>[10x]DYKDDDDK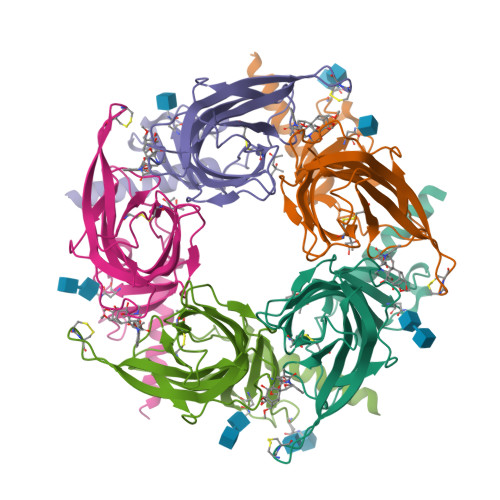LHSQANLMRLKSDLFNRSPMYPGPTKDDPLTVYLSFSLLDIVKADSSTNEVDLVYWEQQSWKLNSLMWDPNEYGNITDFRTSAADIWTPDITAYSSTRPVQVLSPQNALVNSSGHVQYLPAQRLSFMCDPTGVDSEEGATCAVKFGSWSYGGWEIDLKTDTDQVDLSSYYASSKYEILSATQTRSERFYECCKEPYPDVNLVVKFRERRAGNGFFRNLFDSR Banna virus (BAV) is the prototype Seadornavirus, a class of reoviruses for which there has been little structural study. Here, we report atomic cryo-EM structures of three states of BAV virions—surrounded by 120 spikes (full virions), 60 spikes (partial virions), or no spikes (cores). In the full and partial BAV virions, genomic dsRNA segments and a number of RNA-dependent RNA polymerases (RdRps, VP1) are packaged in a double-layered icosahedral capsid consisting of three proteins (VP2, VP8, and VP10). The spikes protruding from the outer capsid shell are heterohexamers composed of a VP4 trimer capped by a VP9 trimer.

Visual inspection and 2D class averaging of purified BAV YN15-126-01 virions on cryo-EM micrographs revealed two types of virions: one surrounded by more spikes on the viral surface (hereafter referred to as full particles), and the other with sparser spiky density (partial particles). In the full BAV virions, there are 60 spikes sitting on VP10A and VP10B, respectively, while in the partial virions, there are only 60 spikes on VP10A. In contrast, in the double-layered full BAV particles, 120 spikes made up of a VP4 trimer (for membrane penetration) and VP9 (for receptor binding) emanate from VP10 located at both type II and type III channels. Local reconstructions focused on the fivefold vertices produced a clear map at 2.6 Å resolution for tracing most residues of VP2, VP4, VP8, and VP10 in the icosahedral asymmetrical unit (ASU). VP4 trimers are situated in the cavity formed by six VP8 trimers and directly interact with VP10A or VP10B. The C3 symmetry is broken for the three N-terminal tails (various numbers of residues were traced) within one VP4 trimer, which are involved in forming the asymmetric interface between the VP4 trimer and VP10 monomer. Despite the symmetry mismatch between the VP4 trimer and VP10 monomer, the interface is similar for VP10A and VP10B. The VP4 trimer has an overall negatively charged patch near its C3 axis at the VP4–VP10 interface, while positively charged residues R65 and R121 are present on the VP10 side. At physiological pH, VP4 (pI = 5.9, negatively charged) would electrostatically interact with the basic VP10 protein (pI = 9.0), suggesting that electrostatic interactions between the VP4 trimer and VP10 may play an important role in association of spikes on the virus surface. Binding of VP4 trimers also results in a total ~1800 Å2 of buried surface area on VP8 molecules surrounding VP10A, which is ~10% more than for VP8 surrounding VP10B ( ~ 1600 Å2), likely contributing to different affinity of VP4 trimers for the outer capsid shell in the full BAV particles.

>MPRKKDQVTKNDDGNQTSDVQTQDFKTAVQPDTNTAQLIKTYSNPKQRGDKGEIIYDGGLSSKLADVVDKTTEPHNADGAVKDGRIAPVKLDLEKQKLDKLKLFETSPFDPLTIKNNQDVVDKLYATQSSSIQEVVPTKTFATELQFGVTSEDMAKIYGAVAAVSKNVNSSVTYEVKRGTHELIKVPTIPHNLVLIQSDNGKHALIKEDLGQWPVETGISLVNQAGVFAVQLANKLGIDKPFVLDAGSNYFTDTSFIDTRKYCTDGLSPREIQKALNRQRAYYDRPELTISENKTLLSQSIIYPDADGNDVSIIFSGAMSHAIFTYAQSQWNKNIIKLDDYIREITLTVPKQYRPRRFKEIEHTHGYVYRELNQGSLLPLVDANLKESSSYYFKKLMSSISNVPVDARTLQSATAALAADTGQAVNRAQHVSMLTNRLTTANAPTVRAITVLTCMFKQFRIGMTYALDPNIMDVAAATCMLLFRPAQSISDEQYRYCLQTMAVFLTNTTYDIVNNDTIDVLKMKLRNQGWPFVERYNAVEIDMSVEPLRSPGQVGRYYNPFNIDPLTKKHVEDRLEEFINQVQVGRFRNASGNAVGTTLAAFLRACRDKTSANWRGYSVLVSRYRSLIPNELFESLRNISGEYNINPQDEHSFFFALAQINADDEFIGAIDKESAEYLDEYATLARDISNSLTLVKAAFGPLERTSGSIINHANNLNKVINHVFADKPLISETMLKILTIDGTTGKDGYRNWLDKLVGHNYPVYVEPVVNIMNFISARFVADSSYFGYTNEIMIMPNHINVPVDDRFGFRDSPFCTSLPRTIMGNDVRRISYNVFSMMEDIDDVISEGFILYDAYFNFSYDIMTTDGVTRLKEDILIVTDTGNDIKPIHFYIYFENRNDKKLRYESKMNVSYRLYIKTPACLLPLSDYMRAQHDYVSPSSSRVYIKDPAVVYTRS[2x];>MANRATSAFLDNPHPVGVNYVDEGSRQFVAVAELLASKLIDSSRESDESNSDVPFVQAYSKFADDNPRHLRVKTGGKMANALTNVIRSYYSINAPAIVPQVEIDRLASKATVSGDMYNSYAIFNSVPIVEVLSPARTTVSIVGSDRADVTMLNTGAGAANITFNFGQIAETVILKGSVPFQLARLNQPMPAARFTYKLRPLDGPFIVVLPVGNPLVISATAATRIQVPLAFNKALVESGFQTAMNDGLFDIQNVNYYSSFDEFIISQYHAQDGINRVSTCVILGLALQAYDQMRRALPVRRV[13x];>[2x]MDVLSKGSLKELLAHLEKTPLEEAISYRIGTVPYQNVLISRNEYYNQLYPDTTSLIDGVSREGQRNVNGLIMSIISYVVSGSGHYIPNIGFMLLRRSILDILTKHDTGLVTNNLNYGIIARNLTVSKMNCEQRKRMLICFKLLAYKDGNQNDYEIYLNQNIPLKQIAPNFIPGDMRTVIHNQDQLAIVGIPAYRLTQSTELSIRDDNAKSYKLGYVDWYNSNSFLRERSEFNLIRLKDRDTKYGKLNGW;>[6x]MAWVTQAYSSGLSQNSIISLTGNDRTVADGTFNSMIMPRAVIANEREHFMKTRIDKIEHDLNRSAKQEMMDRQSLAEDYNALNLAVGQEIKLDIATQHQLNRLGSAMYKADHERETELTDLINRIRENEVTVNGILENQKAITAAERADLLLEVVASTAKSVSAAGRAAADGSGVVPVFGPSVANGIKVGIDIADSVAEAAIAVKESGIITQLNDVYHAFQSVHVAPNDVIKPAAVVAGTSTELIGNLQAIYSRLRSHSDIGFKKATVGDVIPNSYMIKPVNSTEYASWQLYVIHPVQGSLGLVVQLMGDALTYNVFAQYGNTSASEFGKTVLTGGATNTALEGTKVKFQTKVTAQQALALTMALKDAASMLSQGELIGYFEQYINLALEPDNLSLQDNMHKYHHLLTSQNSPIDWNYHDEEMHKWLDSRKTTNYDAMQKKDGTVIADIHIPKVFNDLRNTTLHCKLEGKQTIAGYTVYEYLIGPWAHYGDIDYSVVVDTLNEETKWYCEVIGIDGHLLIEKSVQHKPEKILELTVNDSGVTSFNGRNHDRLKLKVYVKDSLSVKVFRNWIGINAPRVKTKMFNDHIGVKYDYSHFDKNISPAHLTLTDLGWHTWDQYNAGNWTNIKP;>[6x]MLSETELRALKKLSTTTSRVVGDSTLALPSNVKLSKGEVEKIAVTKKEMFDELAQCNLPTIELITREHTFNGDVIRFAAWLFLMNGQKLMIANNVAVRMGMQYATNLAGNNVKITYVTSNNVVKLGHIAAGVLANPYSNKGSGLFITYEYNLISNLIETGKVCVLFITSLSTTASSTNSFAYSTCSVPIENWDFNMIKLTAETSCASLTAMTNLVNSLVPGERTRPVGLYVDIPGVTVTTSASSGSLPLTTIPAVTPLIFSAYTKQVEEVGVINTLYALSYLP> SNYPAYMDNYLKEVINQVEEETGYNLLTTGMDVYTNVDQEAQKHLWDIYNTDEYVAYPDDELQVASTIVDVSNGKVIAQLGARHQSSNVSFGINQAVETNRDWGSTMKPITDYAPALEYGVYESTATIVHDEPYNYPGTNTPVYNWDRGYFGNITLQYALQQSRNVPAVETLNKVGLNRAKTFLNGLGIDYPSIHYSNAISSNTTESDKKYGASSEKMAAAYAAFANGGTYYKPMYIHKVVFSDGSEKEFSNVGTRAMKETTAYMMTDMMKTVLTYGTGRNAYLAWLPQAGKTGTSNYTDEEIENHIKTSQFVAPDELFAGYTRKYSMAVWTGYSNRLTPLVGNGLTVAAKVYRSMMTYLSEGSNPEDWNIPEGLYRNG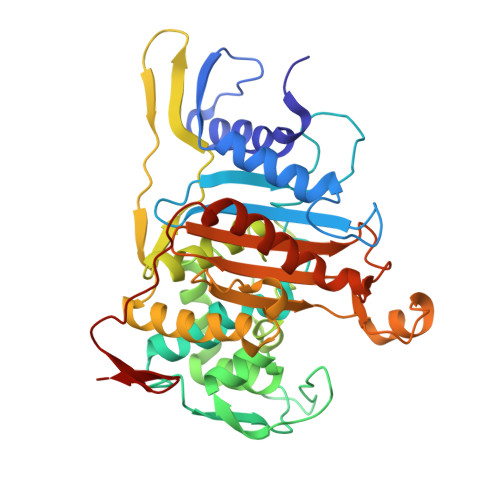EFVFKN> ADVAGTSNRDFRGREQRLFNSEQYNYNNSLNGEVSVWVYAYYSDGSVLVINKNSQYKVGISETFKALKEYREGQHNDSYDEYEVNQSIYYPNGGDARKFHSNAKPRAIQIIFSPSVNVRTIKMAKGNAVSVPDEYLQRSHPWEATGIKYRKIKRDGEIVGYSHYFELPHEYNSISLAVSGVHKNPSSYNVGSAHNVMDVFQSCDLALRFCNRYWAELELVNHYISPNAYPYLDINNHSYGVALSNRQ

Here, we have developed a cell-free protein crystallization (CFPC) method, which involves direct protein crystallization using cell-free protein synthesis. We have succeeded in determining crystal structures of two types of proteins with high-resolution using CFPC. The polyhedra crystal (PhC) produced in insect cells by infection of cypovirus (cytoplasmic polyhedrosis virus, CPV) is one of the most highly studied in-cell protein crystals. The structure of crystalline inclusion protein A (CipA), a bacterial in-cell crystal, had not been previously reported.

We have succeeded in crystallization and structure determination of nano-sized polyhedra crystal (PhC) at a high resolution of 1.80 Å. A 20 μL reaction mixture containing 10 μL of WEPRO®7240 and 10 μL of the mRNA solution was overlaid with a 200 μL SUB-AMIX® SGC solution in a 1.5 mL microtube and then incubated at 20 °C for 24 h. The crystals prepared from the CFPC reaction (PhC_CF) have the same cubic morphology as that of PhC synthesized in insect cells (PhC_IC). The average size of PhC_CF (580 nm) is approximately one-fifth of that of PhC_IC (2700 nm) as determined by scanning electron microscopy (SEM). To collect diffraction data from the nano-sized PhC_CFs, the crystals isolated from the reaction mixture were diffracted using the micro-X-ray beam of the BL32XU beamline equipped with Serial Synchrotron Rotation Crystallography (SS-ROX) at SPring-8. The root mean square deviation (RMSD) value of the Cα atoms for the structure from PhC_IC is 0.09 Å. The main difference between PhC_CF20°C/24h and PhC_IC is that PhC_CF20°C/24h shows no electron density of nucleotide triphosphates (NTPs) bound to the monomer interface, which are observed in PhC_IC. The average B-factor values per residues of all atoms in PhC_CF20°C/24h show a large value for His76 because of the lack of cytosine triphosphate (CTP) interacting with His76 in PhC_IC. In PhC_IC, the amino acid residues surrounding guanine triphosphate (GTP) and adenosine triphosphate (ATP) interact with the NTPs, but in PhC_CF20°C/24h, which lacks these electron densities, there is no significant difference in the side chain conformation between PhC_CF20°C/24h and PhC_IC. These results indicate that the NTP binding is not essential for the crystallization of PhM.> MEAGITGTWYNQLGSTFIVTAGADGALTGTYVTARGNAESRYVLTGRYDSAPATDGSGTALGWTVAWKNNY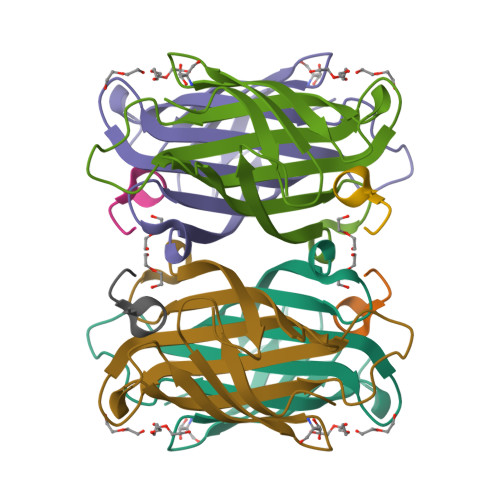RNAHSATTWSGQYVGGAEARINTQWLLTSGTTEHWYSTLVGHDTFTKVKPSAAS;> XSAWSHPQFEKX> GDDEELQSQYGYVQFKLYKSTSFEKGTTTRAVGKLESMSSAQKIKVVMTHNGTTVSQTLLLNAYNANNAEYGLRSDKLQLLAGTYKIVGYYLYDGLDEVLLAGPAG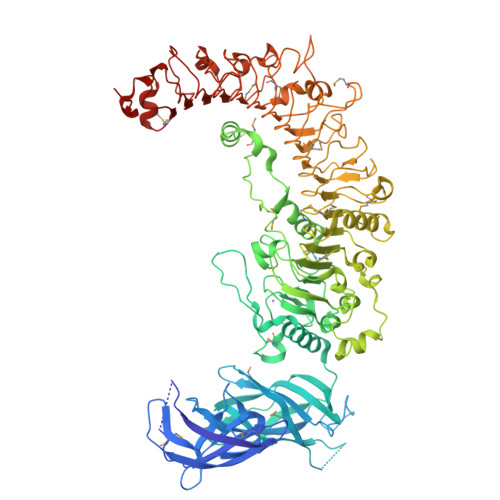DDNELTVVSGGLLEKALTVDAVPHGTVTFKLSKEGISTRAAGEYLFSNIRYVDVTVMNSFNRVTTELKGMKVTYKEDSKEHQNPDNANDKYMDIGVATCDSAVWLPAGTYQVVAYTTYSQSGIKRSELETQSVRGESFTVIDNKLTKDANVPIQLKETAEYIKDYKALKAIWEALDGKNWRYYSGTINNTIHSLNWNFNKELDMWGDQPGVDLDNNGRVTGLSLAGFGAKGRVPDAIGQLTELKVLSFGTHSETVSGRLFGDEELTPDMSEERKHRIRMHYKKMFLDYDQRLNLSDLLQDAINRNPEMKPIKKDSRISLKDTQIGNLTNRITFISKAIQRLTKLQIIYFANSPFTYDNIAVDWEDANSDYAKQYENEELSWSNLKDLTDVELYNCPNMTQLPDFLYDLPELQSLNIACNRGISAAQLKADWTRLADDEDTGPKIQIFYMGYNNLEEFPASASLQKMVKLGLLDCVHNKVRHLEAFGTNVKLTDLKLDYNQIEEIPEDFCAFTDQVEGLGFSHNKLKYIPNIFNAKSVYVMGSVDFSYNKIGSEGRNISCSMDDYKGINASTVTLSYNEIQKFPTELFATGSPISTIILSNNLMTSIPENSLKPKDGNYKNTYLLTTIDLRFNKLTSLSDDFRATTLPYLSNMDVSYNCFSSFPTQPLNSSQLKAFGIRHQRDAEGNRILRQWPTGITTCPSLIQLQIGSNDIRKVDEKLTPQLYILDIADNPNISIDVTSVCPYIEAGMYVLLYDKTQDIRGCDALGIER>[2x]GN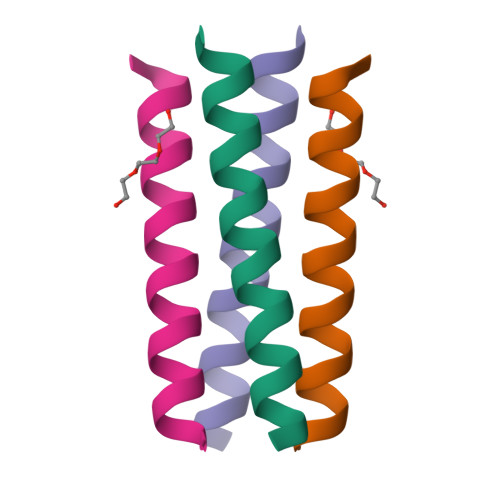ADELYKELEDLQERLRKLRKKLRSG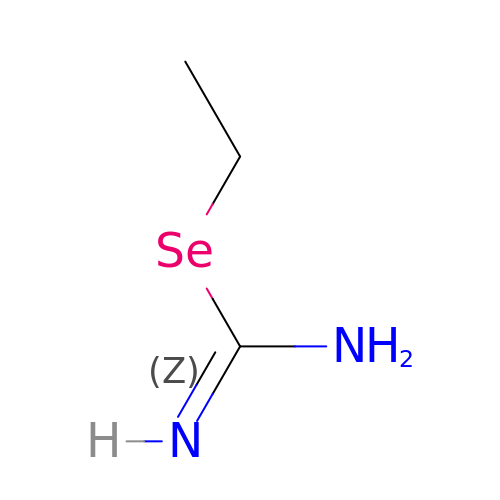SE-ETHYL-ISOSELENOUREA | C3 H8 N2 Se | FFKYNFXDBBLWGF-UHFFFAOYSA-N>MGSSHHHHHHSQDLDEVDA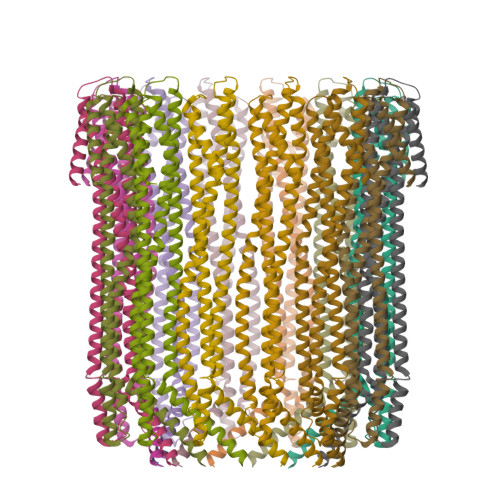GSMTEIVADKTVEVVKNAIETADGALDLYNKYLDQVIPWQTFDETIKELSRFKQEYSQAASVLVGDIKTLLMDSQDKYFEATQTVYEWCGVATQLLAAYILLFDEYNEKKASAQKDILIKVLDDGITKLNEAQKSLLVSSQSFNNASGKLLALDSQLTNDFSEKSSYFQSQVDKIRKEAYAGAAAGVVAGPFGLIISYSIAAGVVEGKLIPELKNKLKSVQNFFTTLSNTVKQANKDIDAAKLKLTTEIVAIGEIKTETETTRFYVDYDDLMLSLLKEAAKKMINTCNEYQKRHGKKTLFEVPEV[14x]>MQNITQSWFVQGMIKATTDAWLKGWDERNGGNLTLRLDDADIAPYHDNFHQQPRYIPLSQPMPLLANTPFIVTGSGKFFRNVQLDPAFNLGIVKVDSDGAGYHILWGLTNEAVPTSELPAHFLSHCERIKATNGK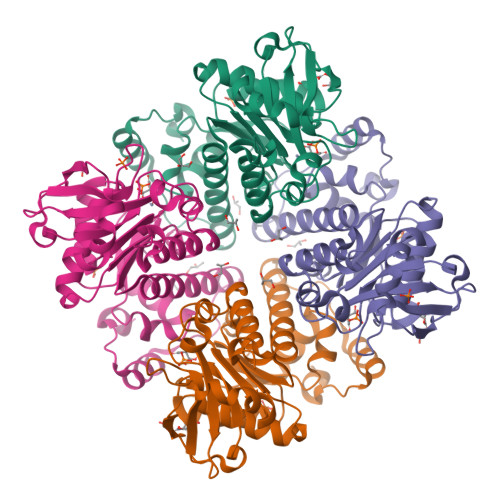DRVIMHCHATNLIALTYVLENDTAVFTRQLWEGSTECLVVFPDGVGILPWMVPGTDAIGQATAQEMQKHSLVLWPFHGVFGSGPTLDETFGLIDTAEKSAQVLVKVYSMGGMKQTISREELIALGKRFGVTPLASALAL[4x]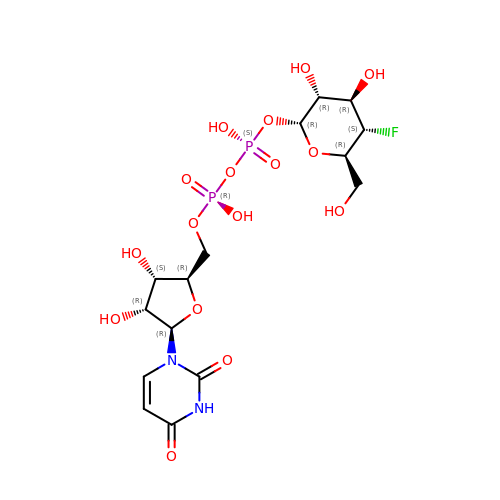URIDINE-5'-DIPHOSPHATE-4-DEOXY-4-FLUORO-ALPHA-D-GALACTOSE | C15 H23 F N2 O16 P2 | OAPPZHVTNHJVAL-JZMIEXBBSA-N> EFPEITEEMEKEIKNVFRNGNQDEVLSEAFRLTITRKDIQTLNHLNWLNDEIINFYMNMLMERSKEK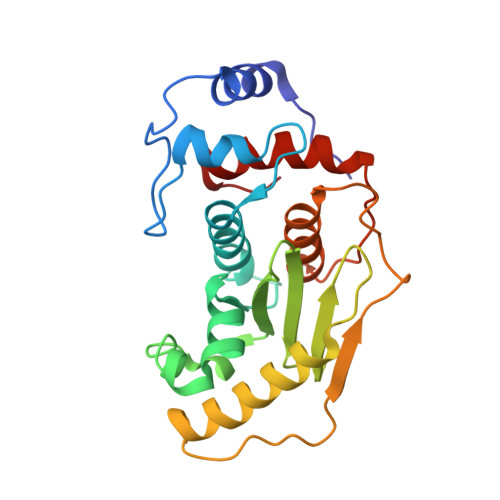GLPSVHAFNTFFFTKLKTAGYQAVKRWTKKVDVFSVDILLVPIHLGVHWCLAVVDFRKKNITYYDSMGGINNEACRILLQYLKQESIDKKRKEFDTNGWQLFSKKSQIPQQMNGSDCGMFACKYADCITKDRPINFTQQHMPYFRKRMVWEILHRKLL>[3x]GAASMEKELRSTILFNAYKKEVFTTNTGTKSLQKRLRSNWKIQSLKDEITSEKLIGVKLWITAGPREKFTAAEFEVLKKYLDSGGDILVMLGEGGESRFDTNINFLLEEYGIMVNNDAVVRNVYYKYFHPKEALVSD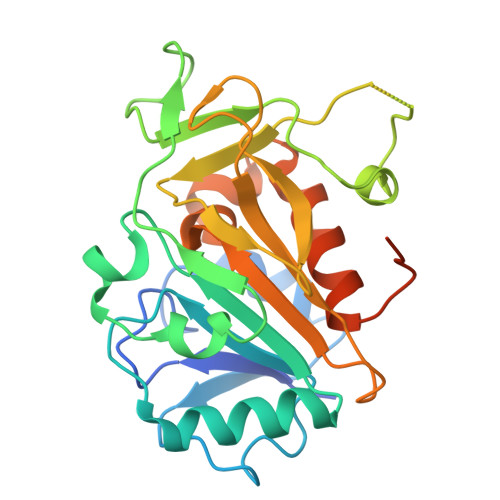GVLNREISRAAGKAVPGVIDEENSGNNAQALTFVYPFGATLSVMKPAVAVLSTGSVCFPLNRPILAFYHSKNQGFGKLAVLGSCHMFSDQYLDKEENSKIMDVVFQWLTTGDIHLNQIDAEDPEISDYTMVPDTA Cyclic GMP–AMP synthase (cGAS) is a cytosolic DNA sensor that produces the second messenger cG[2′–5′]pA[3′–5′]p (2′3′-cGAMP) and controls activation of innate immunity in mammalian cells. Here we show that cGAS-like receptors (cGLRs) are innate immune sensors that are capable of recognizing divergent molecular patterns and catalysing synthesis of distinct nucleotide second messenger signals. In support of this conclusion, Hartmann, Imler, Cai and colleagues have identified cGLR2 as a second functional cGLR in Drosophila and have demonstrated in vivo that cGLR1 and cGLR2 have discrete roles in Drosophila immunity. Together, our results define cGLRs as receptors in animal cells that are capable of detecting diverse pathogen-associated molecular patterns and dictating response to the foreign environment.

To define the function of cGAS-like enzymes in animals, we screened predicted cGAS homologues for suitability in structural analysis and determined a 2.4 Å crystal structure of the human protein MB21D2 (hMB21D2; encoded by C3orf59) and a 1.6 Å crystal structure of a protein from the beetle species Tribolium castaneum (GenBank XP_969398.1). Despite divergence in the primary sequence, the hMB21D2 and T. castaneum XP_969398.1 structures each reveal close homology to human cGAS with a shared bi-lobed architecture, a caged nucleotidyltransferase core, a Gly-[Gly/Ser] activation loop and a putative catalytic triad. A conserved groove is present in both the hMB21D2 and the T. castaneum XP_969398.1 structures, but is notably distinguished by the absence of a Zn-ribbon and the insertion of a C-terminal α-helix in hMB21D2. We hypothesized that the remodelling of this groove controls the detection of distinct ligands. The hMB21D2 surface is overall neutral with no obvious capacity to bind nucleic acids, and no enzymatic activity was detected with a panel of potential activating ligands. Our structural analysis also reveals that the human cGLR MB21D2 is competent for synthesis of nucleotide second messengers and has a remodelled ligand-binding groove that is probably adapted for detection of an unknown stimulus. Together with the known high frequency of hMB21D2 mutations in cancer, these results support a more extensive role for cGLR signalling in human biology.

>SSGARVEELNKLIQEFTKHDQREYDDQRALEIHTAKDFIFSMLGMVQKLDQKLPVANEYLLLSGGVREGVVDLDLDELNVYARGTDYDMDFTLLVPALKLHDRNQPVTLDMRHSALCHSWLSLRLFDEGTISKWKDCCTIVDHINGATNYFFSPTKVADWFYDSISIVLSEIQKKPQRGMPKVEKVEKNGTIISIILGVGSSRMLYDIVPVVSFKGWPAVAQSWLMENHFWDGKITEEEVISGFYLVPACSYKGKKDNEWRLSFARSEVQLKKCISSSLMQAYQACKAIIIKLLSRPKAISPYHLRSMMLWACDRLPANYLAQEDYAAHFLLGLIDDLQHCLVNKMCPNYFIPQCNMLEHLSEETVMLHARKLSSVRSDPAEHLRTAIEHVKAANRLTLELQRRGSTTSIPSPQSDGGDPNQPDDRLAKKLQQLVTENPGKSISVFINPDDVTRPHFRIDDKFF[2x]> EPEFPHNAIEPCVICQTRPKNGCIVHGKTGHLMACFTCAKKLKK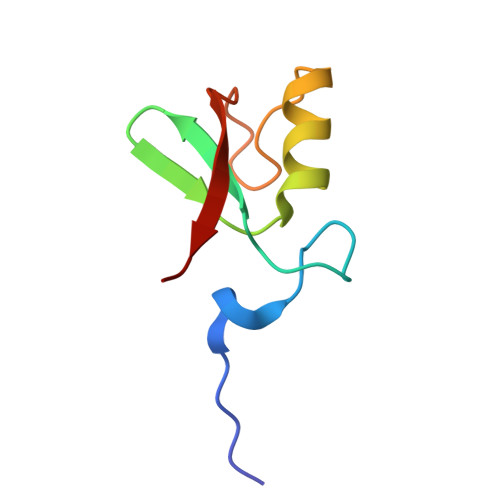RNKPCPVCRQPIQMIVLTYFP> DDKMDYDFKVKLSSERERVEDLFEYEGCKVGRGTYGHVYKAKRKDGKDDKDYALKQIEGTGISMSACREIALLRELKHPNVISLQKVFLSHADRKVWLLFDYAEHDLWHIIKFHRASKANKKPVQLPRGMVKSLLYQILDGIHYLHANWVLHRDLKPANILVMGEGPERGRVKIADMGFARLFNSPLKPLADLDPVVVTFWYRAPELLLGARHYTKAIDIWAIGCIFAELLTSEPIFHCRQEDIKTSNPYHHDQLDRIFNVMGFPADKDWEDIKKMPEHSTLMKDFRRNTYTNCSLIKYMEKHKVKPDSKAFHLLQKLLTMDPIKRITS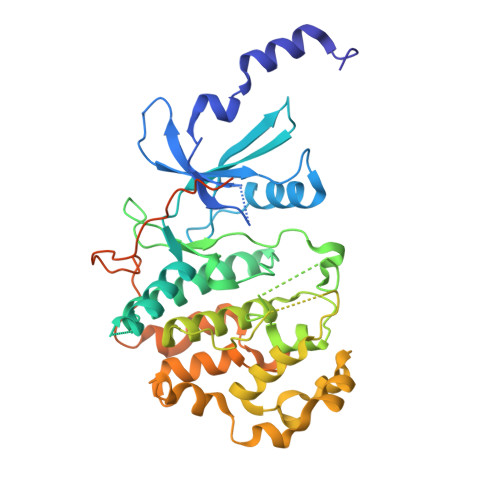EQAMQDPYFLEDPLPTSDVFAGCQIPYPKREFLTEEEPDDKGDKKNQQQQQGNNHTNGTGHPGNQDSSHTQGPPLKK>MGSSHHHHHHSQDPMKVIFFSMHPYEEEFLGPILPSDWDVEMTPDFLDETTVEKAKGAQVVSLFVSDKADGPVLEALHSYGVGLLALRSAGYDHIDIETAKRLGIKVVNVPAYSQHAIADHTLAIMLALIRRLHRAHDKVRLGDFDLDGLMGFDLNGKVAGVIGLGKIGRLVATRLKAFGCKVLGYDPYIQPEIVENVDLDTLITQADIISIHCPLTRENFHMFNEETFKRMKPGAILVNTARGGLIDTKALLEALKSG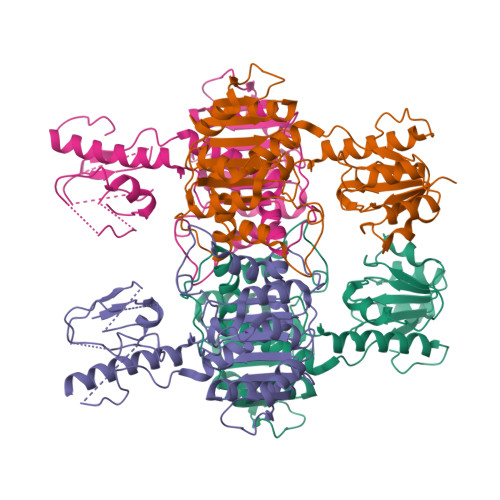KLGGAALDVYEYERGLFFKNHQKEGIKDPYLAQLLGLANVVLTGHQAFLTREAVKNIEETTVENILEWQKNPQAKLKNEI[4x]>MSNFLDLQKQRRSIYALGKTVDLSKAELVALIQNAIKQAPSAFNSQTSRALVLFGQDSQDFWNKIAYSELEKVTPAEAFAGTKAKLESFAAGVGTILLFEDQAVVRNLEENFPLYAENFQPWSEQAHGIALYAIWLALAEQNIGMSVQHYNPLVDA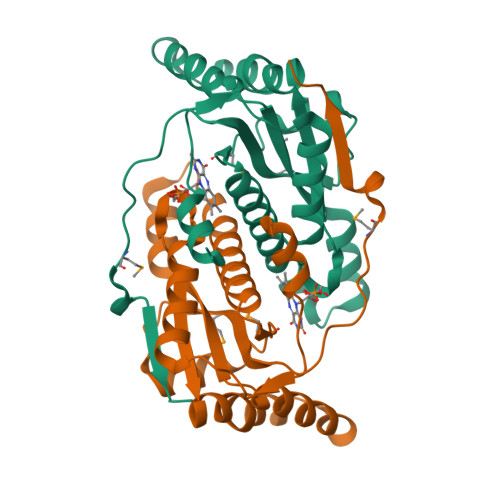QVAEKYDLPTNWKMRAQIPFGSIEAPAGEKEFMADQERFKVFGDLEHHHHHH[6x]> MTDNHIDVLINGCGIGGAMLAYLLGRQGHRVVVVEQARRERAINGADLLKPAGIRVVEAAGLLAEVTRRGGRVRHELEVYHDGELLRYFNYSSVDARGYFILMPCESLRRLVLEKIDGEATVEMLFETRIEAVQRDERHAIDQVRLNDGRVLRPRVVVGADGIASYVRRRLLDIDVERRPYPSPMLVGTFALAPCVAERNRLYVDSQGGLAYFYPIGFDRARLVVSFPREEARELMADTRGESLRRRLQRFVGDESAEAIAAVTGTSRFKGIPIGYLNLDRYWADNVAMLGDAIHNVHPITGQGMNLAIEDASALADALDLALRDACALEDALAGYQAERFPVNQAIVSYGHALATSLEDRQRFAGVFDTALQGSSRTPEALGGERSYQPVRSPAPLG

In this study, we show that the catalytic activity of the flavoprotein monooxygenase (FPMO) PqsL can be triggered by blue-light illumination. The enzyme is involved in the biosynthesis of 2-alkyl-4-hydroxyquinoline N-oxides (AQNO) in the opportunistic pathogen Pseudomonas aeruginosa. It is homologous to group A FPMOs13 and has a relatively high similarity to p-hydroxybenzoate hydroxylase (pHBH), the most thoroughly studied FPMO14. In contrast, PqsL catalyzes the hydroxylation of an aromatic-amine group, a rather uncommon reaction, and remarkably shows no intrinsic catalytic activity with NAD(P)H as cosubstrate.

Crystallization experiments with wild-type PqsL produced crystals of very high quality. This allowed us to solve the three-dimensional structure of the enzyme bound to FAD and its substrate 2-ABA at 1.8 Å resolution. We therefore focused our analysis on the specific properties of PqsL’s catalytic site where a molecule of 2-ABA could be located based on the electron density map. 2-ABA occupies a large cavity above the edge of the flavin ring. Specifically, 2-ABA interacts with the main chain atoms of two active-site loops (residues 46–48 and 300–303) and its carboxylate group H-bonds to the backbone nitrogen of Asp47 and a water molecule. A critical observation was that the substrate aromatic ring is oriented with its amino group pointing away from the flavin. This binding orientation cannot sustain catalysis because the amino group must be in reach of the terminal oxygen of the flavin-hydroperoxide intermediate. A simple 180° flipping rotation around the C1–C4 axis of the aromatic ring would position the amino group of the 2-ABA substrate toward the flavin, in the position expected for amine hydroxylation. The crystallized 2-ABA-stabilized oxidized PqsL could therefore be the dominant enzyme-substrate-inhibitor complex, with a KD of 38.44 ± 3.98 µM. By comparison with the pHBH crystal structures, the flavin in PqsL can be described as in the OUT conformation. The shift of this loop, caused by a kink at the Cα of Tyr276, positions Pro273 of PqsL (Pro267 in pHBH) in direct contact with the flavin, which thereby remains more buried within the protein compared to pHBH.> PKCMIFCPVAATPAQQDALLKDAEKAVADALGKPLSYVMVGYSQTGQMRFGGSSDPCAFIRVASIGGITSSTNCKIAAALSAACER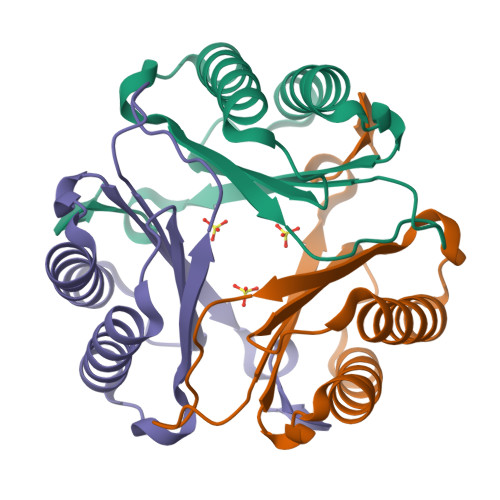HLGVPKNRIYTTFTNKSPSEWAMGDRTF> MSFNESASIPTGLTYDDVLIIPQHSRVTSRKEVNTTTRLSRNVKLSIPIVASNMDTVCEQRMAVAMAREGGIGILHRFCSIEEQCAMLREVKRAQSFLIESPRIILPHETAREAWEGLNWKGRVGGVGCLLVVNCKNERKLLGIITRHDLKLADESTTVESLMTPVDKMVVSTNTSISLEEVTHLMRKGRTANVPIVGQNGQLLYLVTLSDVVKLRKNKQASLDSRGRLLVGAAVGVKKDDMNRAIRLVEAGADVLVVDIAHGHSDLCINMVKRLKGDPRTASVDIIAGNIASAEAAEALIDAGADGLKIGVGPGSICITRLVAGAGVPQLSAVLACTRVARRRGVPCIADGGL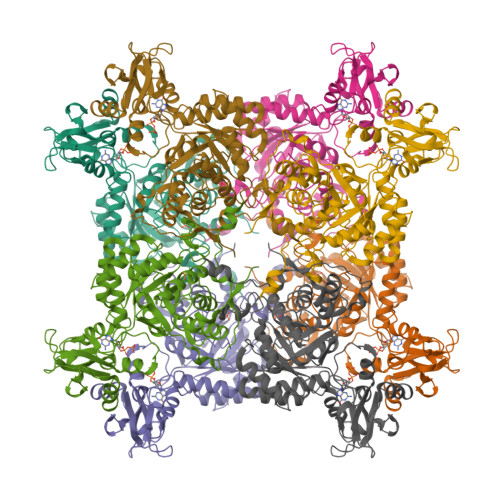RTSGDISKAIGAGADTVMLGNMLAGTDEAPGRVLVKDGQKVKIIRGMAGFGANLSKAERERTQDEDVFSSLVPEGVEGSVACKGPVGPIVRQLVGGLRSGMSYSGAKSIEEMQRRTRFVRMTGAGLRESGSHGVAKLKLAAALEHHHHHH>[2x]GAGSTAGKVIKCKAAVLWEEKKPFSIEEVEVAPPKAHEVRIKMVATGICRTDDHVVSGTLVTPLPVIAGHEAAGIVESIGEGVTTVRPGDKVIPLFTPQCGKCRVCKHPEGNFCLKNDLSMPRGTMQDGTSRFTCRGKPIHHFLGTSTFSQYTVVDEISVAKIDAASPLEKVCLIGCGFSTGYGSAVKVAKVTQGSTCAVFGLGGV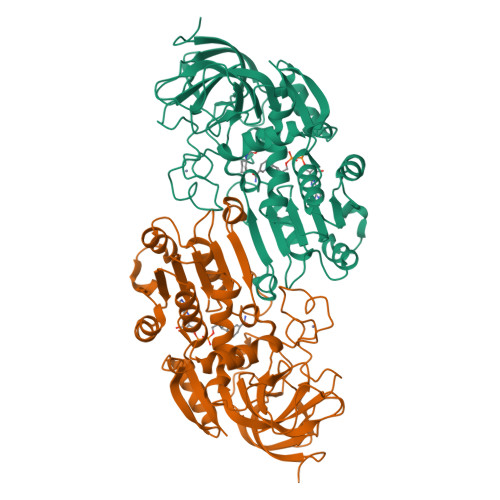GLSVIMGCKAAGAARIIGVDINKDKFAKAKEVGATECVNPQDYKKPIQEVLTEMSNGGVDFSFEVIGRLDTMVTALSCCQEAYGVSVIVGVPPDSQNLSMNPMLLLSGRTWKGAIFGGFKSKDSVPKLVADFMAKKFALDPLITHVLPFEKINEGFDLLRSGESIRTILTF> SIAGTVMDHDKIAKLPASGSPLETKFQPQLHIGNGCHSYPAVDAQGNWSGGLKPTGAPSAACKD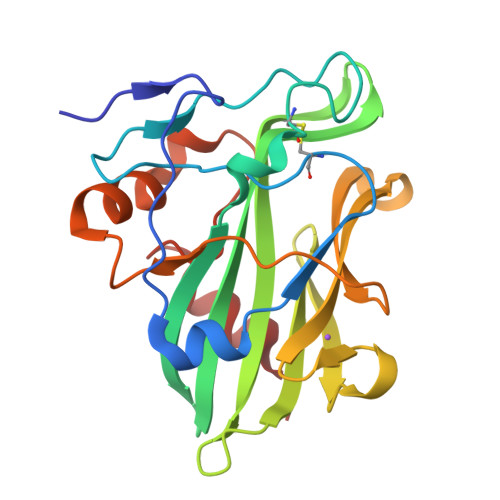TSKAQTYVRSATFQGKTALVYAWYMPKDEISTGIGHRHDWEGAVVFLNSDTQQIDGVAASAHGKWRKYPNPGGANIDDTHVKLQYSAEPVINSHALDLTDKGGDLPTLASWEGMGADARAAINERSHWGDANPPIADSLIGSSLSGAWMW> GSPEFDSLYPIAVLIDELRNEDVQLRLNSIKKLSTIALALGVERTRSELLPFLTDTIYDEDEVLLALAEQLGTFTTLVGGPEYVHCLLPPLESLATVEETVVRDKAVESLRAISHEHSPSDLEAHFVPLVKRLAGGDWFTSRTSACGLFSVCYPRVSSAVKAELRQYFRNLCSDDTPMVRRAAASKLGEFAKVLELDNVKSEIIPMFSNLASDEQDSVRLLAVEACVNIAQLLPQEDLEALVMPTLRQAAEDKSWRVRYMVADKFTELQKAVGPEITKTDLVPAFQNLMKDCEAEVRAAASHKVKEFCENLSADCRENVIMSQILPCIKELVSDANQHVKSALASVIMGLSPILGKDNTIEHLLPLFLAQLKDECPEVRLNIISNLDCVNEVIGIRQLSQSLLPAIVELAEDAKWRVRLAIIEYMPLLAG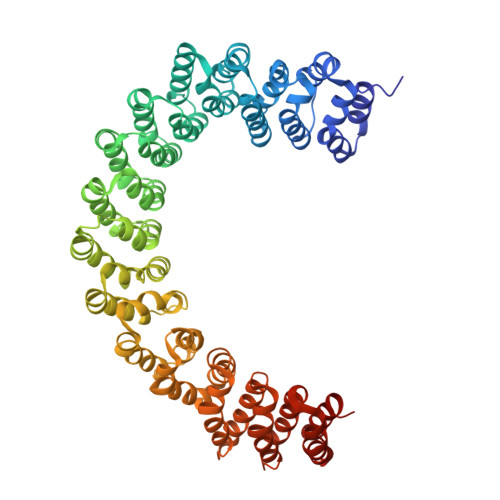QLGVEFFDEKLNSLCMAWLVDHVYAIREAATSNLKKLVEKFGKEWAHATIIPKVLAMSGDPNYLHRMTTLFCINVLSEVCGQDITTKHMLPTVLRMAGDPVANVRFNVAKSLQKIGPILDNSTLQSEVKPILEKLTQDQDVDVKYFAQEALTVLSLA>[2x]MFEQRVNSDVLTVSTVNSQDQVTQKPLRDSVKQALKNYFAQLN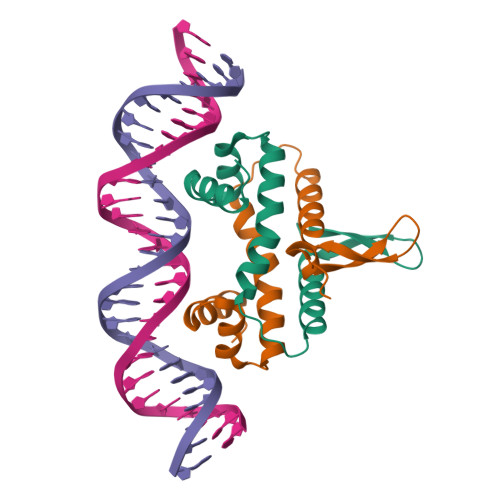GQDVNDLYELVLAEVEQPLLDMVMQYTRGNQTRAALMMGINRGTLRKKLKKYGMN> MYRYEKKGPKRGVALYSYSAEFGLTKTLEDCFEDLHDMGAHGIEILANTHIENYPYPTDEWVEKWWRLCDKYEIVP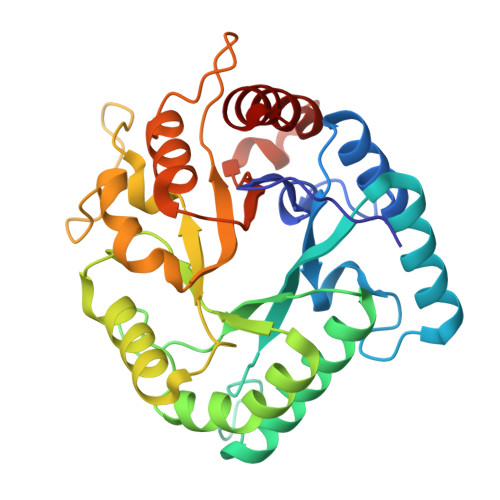VEYGNWIDSHVLGDRDLTTEESVEMLKRDIRLAHRLGFTVMRTKMPVINDLLEPVENWKEIIKGALPLAEELGIKMCPEIHTPSNLKGKLVNDFVEFIKETGTKNFGLNIDFSVFRTSFAEGEWVDPNYTPNKPEDIIPLLPYVYCCHAKFIHMSDDFKETTIPYEEVVKTMEDNGYEGYLLSEYEGADKYDEGYEVGQTLRKHHILLKNLLGD> MLELKFVRNNPDIVGRALISRNMGTELIDSLLEYDAAWRECLIEGDDLKHKRNVVTREIAQLKKENKDAASRINEMQGINSRIKELDDKIRDYKSKINEIMLSIPNIPSETTPVGKDENDNPVVRVVGEPREFTFTPKPHWEIGESLDILDFERAAKISGQGFAVYKGMGAKLERALINFMLDVHTRQGYLEVFPPVLINEKAMTGTGQLPKFKDDMYGCTDGFYLAPTAEVPVTNLFMDEYMENLPVFLTAYTACFRREAGKHGQDTRGIIRNHQFNKVELVKFVMPET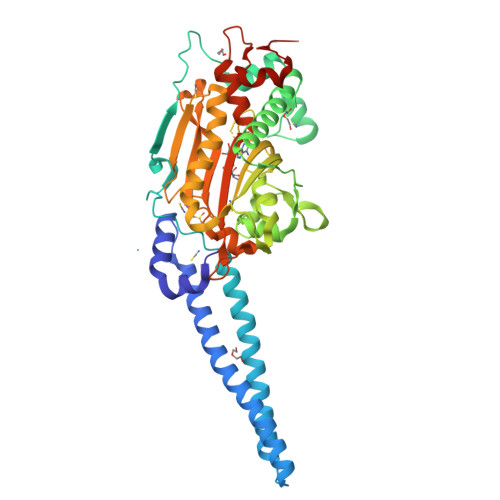SYEELEKLTLDAEEILKLLKLPYRVVSLCTGDLGFSAAKTYDLEVWVPTQEKYREISSCSNFDNFQARRANIRYRTPEGPQFVHTLNGSGLAVGRTVVAILENYQREDGSVVIPEVLRPYMGGAEVIRPEHHHHHH> MTDIYIPPEGLYFRLLGFASRQVIFARNSPSPDVGLSPVNDQATDQYFSLIYGTGEHAGLYAIKSKATGKVLFSRRPAEPYVGQIDGDGRYPDNWFKIEPGKTYLSKYFRLVQPSTGTALVSRTHLQPYFWNHPQTEVFDDQYFTFLFEDMSIDKIEYDLKDGRILSSTPNVLATQTLENTSSQTQEMSF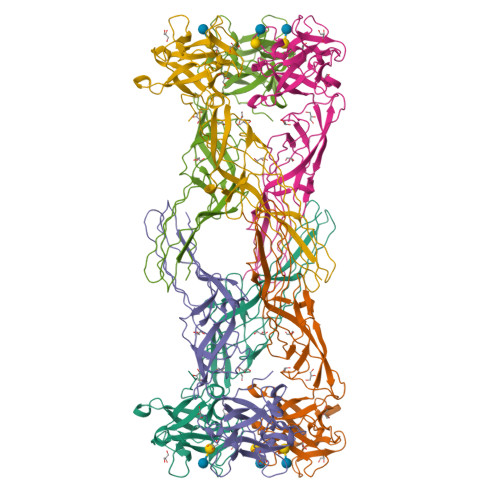NLSQTLTQTSTFAYTAGFTIAVGTAFKAGVPIFAETEFKVDISVDNQWNWGEENTFSKTYTATFSVRAGPGETVKAVSTVDSGIINVPFTAYLSSKSTGFEVTTEGIWRGVSSWDLRHTLTSVTA> PELPEVETIRRTLLPLIVGKTIEDVRIFWPNIIRHPRDSEAFAARMIGQTVRGLERRGKFLKFLLDRDALISHLRMEGRYAVASALEPLEPHTHVVFCFTDGSELRY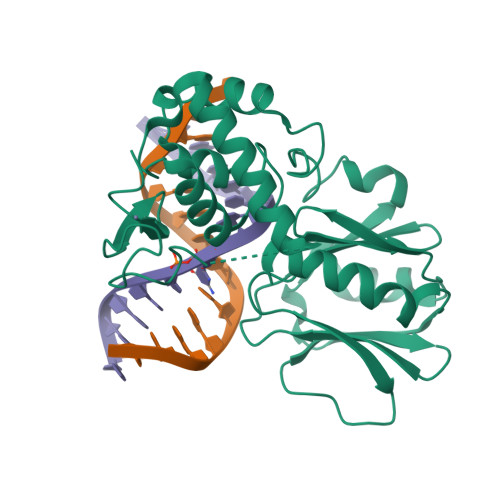RDVRKFGTMHVYAKEEADRRPPLAELGPEPLSPAFSPAVLAERAVKTKRSVKALLLDCTVVAGFGNIYVDESLFRAGILPGRPAASLSSKEIERLHEEMVATIGEAVMKGGSTVRPYVNTQGEAGTFQHHLYVYGRQGNPCKRCGTPIEKTVVAGRGTHYCPRCQR NOD1 and NOD2 (Nucleotide-binding oligomerization domain-containing proteins 1 and 2) are cytosolic receptors of the innate immune system, which respond to intracellular fragments of the bacterial peptidoglycans, D-glutamyl-meso-diaminopimelic acid (iE-DAP) and muramyl dipeptide (MPD), respectively. Upon ligand recognition, NOD receptors oligomerise and recruit an adaptor protein, Receptor Interacting protein kinase 2 (RIP2), through interactions of their respective CARD domains. RIP2 also contains an N-terminal dual-specificity ser/tyr kinase domain (RIP2K), which belongs to the TKL kinase family (Tyrosine kinase-like). RIP2 undergoes auto-phosphorylation and K-63 linked ubiquitination at Lys209, becoming a scaffolding protein for downstream effectors.

To avoid this stability problem, we replaced the conserved lysine with an arginine (K47R) instead of an alanine. RIP2KK47R crystallized in a different space group (P212121) with two quasi two-fold dimers (denoted AB and CD) per asymmetric unit and the structure was refined at 2.6 Å resolution. The inactive state of RIP2K resembles the Src/CDK-like inactive conformation, with the DFG motif in the IN state and the Helix αC outwardly displaced. Helix αC has rotated by ~17 degrees out from its active state position (calculated using the anglebetweenhelices command in Pymol). Due to the consequent rotation of Leu70, the R-spine is broken. Density for almost all the AS was visible showing that it is structured as an α-helix, as described for the inactive states of EGFR-KD and CDK2 and the monomeric BRAF. The AS helix encompasses residues 167–178, thus including the phosphorylation sites Ser174, Ser176 and Ser178 while residues 180–184 remain disordered. Interestingly the helical AS from monomer A in the AB dimer projects outwards towards the active site of the asymmetrically related monomer C from the CD dimer, forming a putative substrate-enzyme phosphorylation complex. Despite the fact that ADP was added in the crystallisation buffer, no nucleotide is bound, probably due to the bulky arginine blocking the ATP binding site and the sulphate rich crystallisation medium. Thus, the asymmetric unit of the RIP2KK47R crystal shows two quasi 2-fold symmetric dimers, with a slightly altered and weaker dimer interface at the N-termini than is observed in the active state.

>GAMAMNGEAICSALPTIPYHKLADLRYLSRGASGTVSSARHADWRVQVAVRHLHIHTPLLDSERKDVLREAEILHKARFSYILPILGICNEPEFLGIVTEYMPNGSLNELLHRKTEYPDVAWPLRFRILHEIALGVNYLHNMTPPLLHHDLKTQNILLDNEFHVKIADFGLSKWRMMSLSQSRSSKSAPEGGTIIYMPPENYEPGQKSRASIKHDIYSYAVITWEVLSRKQPFEDVTNPLQIMYSVSQGHRPVINEESLPYDIPHRARMISLIESGWAQNPDERPSFLKCLIELEPVLRTFEEI[4x]>ETTVKIASDSSYAPFEFQNGQKKWVGIDVDIMQEVAKINDWKLEMSYPGFDAALQNLKAGQVDGIIAGMTITDERKETFDFSNPYYTSALTIATTKDSKLSDYSDLKGKAVGAKNGTAAQTWLQENQKKYGYTIKTYSDGVHMFAALSSGNIAGAMDDVPVISYAMKQGQDLAMNFPSISLPGGYGFAVMKGKNSTLVDGFNKALAEMKSNGDYDKILKKYGITA[2x]

The adenosine triphosphate (ATP)-binding cassette (ABC) importer GlnPQ from Lactococcus lactis has two sequential covalently linked substrate-binding domains (SBDs), which capture the substrates and deliver them to the translocon. GlnPQ is an ABC transporter involved in the uptake of glutamine, glutamic acid, and asparagine and was found to be a robust model protein to study the mechanism of substrate delivery from SBDs to the translocon. SBDs operate in a Venus-fly trap mechanism, where the binding site for a substrate is located between two lobes of an SBD, which is connected by two antiparallel β-strands (the hinge region). We report three high-resolution structures of SBD1, namely, the wild-type SBD1 with bound asparagine or arginine, and E184D SBD1 with glutamine bound.

In addition, it has been shown through uptake experiments that glutamate is transported by both SBD1 and SBD2 domains. The affinity can be easily tweaked by mutagenesis, for example, the double E184D_V185E and the single E184D mutation in the SBD1 domain yield a significantly increased affinity for glutamine (KD of 1.3 ± 0.15 μM and 1.0 ± 0.1 μM, respectively)24. An interesting structural difference is observed when the wild-type (WT) SBD1 is compared with the E184D mutant, which has ∼90-fold increase in the affinity for Gln and an almost 10-fold decrease in affinity for Asn24. The shorter side chain of D184 induces a different orientation of the hydroxyl groups, which mimics D417 in SBD2. Furthermore, the α-amino of the Gln ligand is differently positioned and shows hydrogen bonding to the hydroxyl group of T96 (like 28 in SBD2) and the Oδ2 of D184 (like D417 in SBD2). The hydrogen bonding with the backbone carbonyl of G94 is the same in the SBD1(E184D) mutant and wild-type SBD2 (G326 in SBD2). In asparagine-liganded SBD1, Y38 makes a hydrogen bond to the α-amino group of asparagine, which is different in SBD1(E184D) where the interaction of the α-amino group is made by the Oδ2 of D184 and D183. The herein reported structure of the SBD1 E184D in complex with l-Gln, combined with the MD simulations, explains the change in affinity for Gln when compared to the wild-type protein. While the global architecture of the binding pocket remains unchanged, there are differences in protein–ligand interactions. The shorter side chain of aspartate at position 184 induces a different orientation of the hydroxyl groups creating additional space for glutamine to bind with a high affinity, but almost without any impact on the affinity for asparagine binding.> QEVQTEQVTVAEGGVAEITCRLHQYDGSIVVIQNPARQTLFFNGTRALKDERFQLEEFSPRRVRIRLSDARLEDEGGYFCQLYTEDTHHQIATLTVLVAPENPVVEVREQ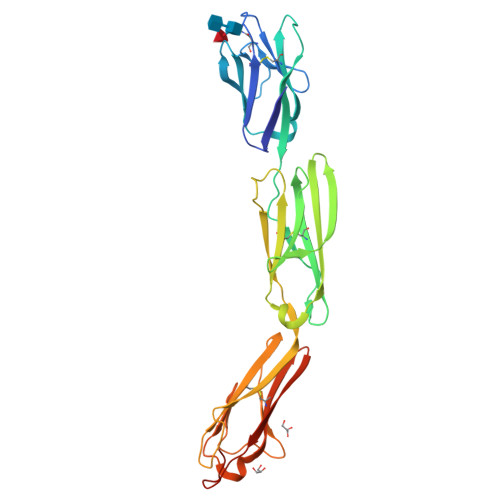AVEGGEVELSCLVPRSRPAAVLRWYRDRKELKGVSSGQENGKVWSVASTVRFRVDRKDDGGIVICEAQNQALPSGHSKQTQYVLDVQYSPTARIHASQAVVREGDTLVLTCAVTGNPRPNQIRWNRGQESLPERAEAVGETLTLPGLVSADQGTYTCEAANKHGHARALYVLVVYDPGAVVEAHHHHHH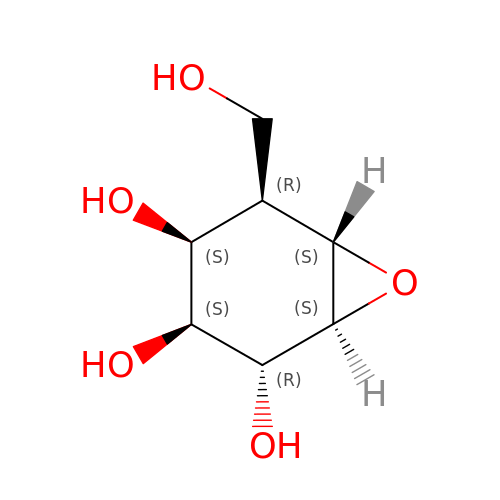(2~{R},3~{S},4~{S},5~{R},6~{S})-5-(hydroxymethyl)-7-oxabicyclo[4.1.0]heptane-2,3,4-triol | C7 H12 O5 | YQLWKYQDOQEWRD-URFJBAFZSA-N> 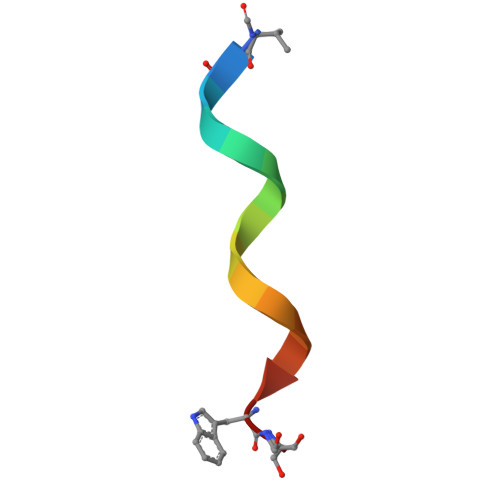VGALAVVVWLYLWLWX Staphylococcus epidermidis expresses glycerol phosphate wall teichoic acid (WTA), but some health care–associated methicillin-resistant S. epidermidis (HA-MRSE) clones produce a second, ribitol phosphate (RboP) WTA, resembling that of the aggressive pathogen Staphylococcus aureus. We report here that the TarM enzyme of HA-MRSE [TarM(Se)] glycosylates RboP-WTA with glucose, instead of N-acetylglucosamine (GlcNAc) by TarM(Sa) in S. aureus. Each blade of the homotrimer contains a catalytic domain with a canonical GT-B fold, consisting of an N-terminal acceptor substrate-binding domain (ABD; residues 1 to 68 and 202 to 302) and a C-terminal nucleotide-binding domain (residues 303 to 492). TarM(Se) is a retaining WTA glycosyltransferase; therefore, the relative positions of donor and acceptor substrates in TarM(Se) and TarP are different.

To understand why the closely related TarM(Sa) and TarM(Se) proteins use different donor substrates, we solved the structure of unliganded full-length TarM(Se) from S. epidermidis at 3.2-Å resolution. Like its homolog TarM(Sa), TarM(Se) forms a symmetric, propeller-like homotrimer, with three blades projecting from the central hub that mediates trimerization via its trimerization domain (TD; residues 69 to 201). In line with this property, the elution profile of TarM(Se) from size exclusion chromatography corresponds to a molecular weight of 162 kDa, suggesting that it exists as homotrimer in solution. On the basis of calibration of the column, TarM(Se) wild-type and TarM(Se)G117R mutant proteins have estimated molecular weights of 162 kDa (N = 6) and 55 kDa (N = 8), respectively, in agreement with the calculated molecular weights of 180 kDa for a TarM(Se) homotrimer and 60 kDa for monomeric TarM(Se)G117R. mAu, milli-absorbance units. Since the resolution of the native TarM(Se) structure was limited to 3.2 Å, we generated a G117R mutant [TarM(Se)G117R]. The C1 hydroxyl group of RboP4 in molecule A is 33.7 Å away from molecule B in the homotrimer, which corresponds to a length of 3.7 RboP units. Therefore, it is not possible that three TarM(Se) molecules in the homotrimer glycosylate the same poly(RboP) chain at the same time in the processive reaction.

>[4x]MKQTYMIVNELDVNKGGMTTAMLTRSKFFLDNEISGDIITFDFKANYKDILKELVQSKKMDKRTQMHNPFIYFKNISNLQHKKYNYTMTRNLSNLLKDSVEIKENSRISRFFNIMSGEYLAYKRETEQETIFDLFKNNLRYKRIYFYKGKIVKTEVFNSDNNLIAEQFYDDNGYLYLYRQINPEKKSIGKTYLVCKEKQFKNNVEFCSYFLDKLIPDINDNIIICDGPGSFPKILKTNHKNVKKFAVIHVNHYKNFDDTGAVKKQEDYILRNANKINGVVMLTEAQKKDIIEKYKITNAYVISNFINITDDYRDKNDNKVVGHISRLVPQKGLPYLIDVAKKVVEQDNSVEFHLYGTGEEKSKIENLIQESNLTNNVKLLGYTTNAIEKIKDFRCVISTSQFEGQGLSLIEAMLLKKPVVAFDVKYGPSDFVKDGKNGYLIENKDIKKMANKILKLLHDKELSKSLGKHGRDTIIDMYQPEKLMVKWKQLFN> AGSHMSKVKVAILGSGNIGTDLMMKLERSNILQLTAMIGIDPESDGLRRAKEKGYTVISTGIKGFLEQPELADIVFDATSAKAHIRHAKLLKEAGKTVLDLTPAAVGALVVPPVNLHKHLDEWNVNLITCGGQATIPIVHAINRVHPVGYAEIVATIASKSAGPGTRANIDEFTQTTARGIEKIGGAKK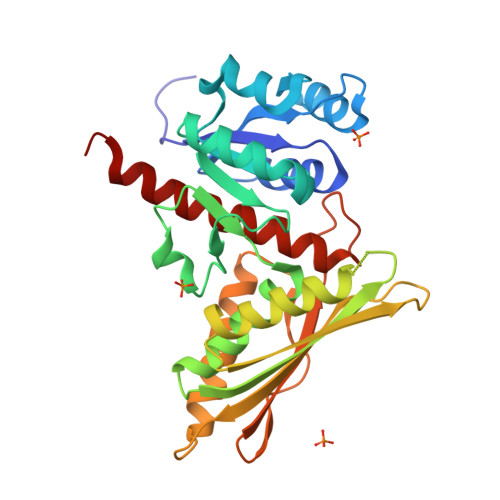GKAIIILNPAEPPIMMRNTVYALVEEGKIDENAIVQSILEMVKTVQSYVPGYRIRTEPIMDGNKITVFLEVEGAGDYLPKYSGNLDIMTAAAVKVAEELAKHKLAAQTA>QAAHLSFARLARRYGDVFQIRLGSCPIVVLNGERAIHQALVQQGSAFADRPSFASFRVVSGGRSMAFGHYSEHWKVQRRAAHSMMRNFFTRQPRSRQVLEGHVLSEARELVALLVRGSADGAFLDPRPLTVVAVANVMSAVCFGCRYSHDDPEFRELLSHNEEFGRTVGAGSLVDVMPWLQYFPNPVRTVFREFEQLNRNFSNFILDKFLRHCESLRPGAAPRDMMDAFILSAEKKAAGDSHGGGARLDLENVPATITDIFGASQDTLSTALQWLLLLFTRYPDVQTRVQAELDQVVGRDRLPCMGDQPN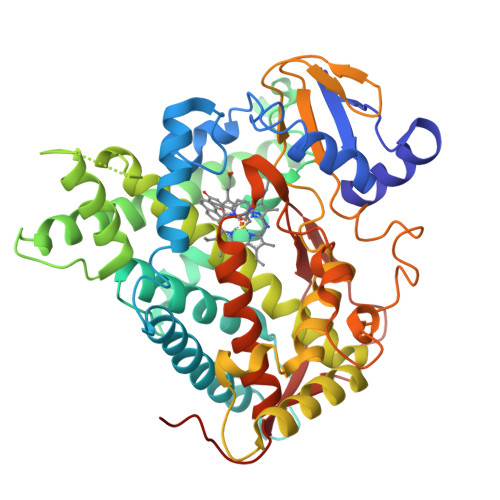LPYVLAFLYEAMRFSSFVPVTIPHATTANTSVLGYHIPKDTVVFVNQWSVNHDPVKWPNPENFDPARFLDKDGLINKDLTSRVMIFSVGKRRCIGEELSKMQLFLFISILAHQCDFRANPNEPAKMNFSYGLTIKPKSFKVNVTLRESMELLD[2x]> GSHMYASLTE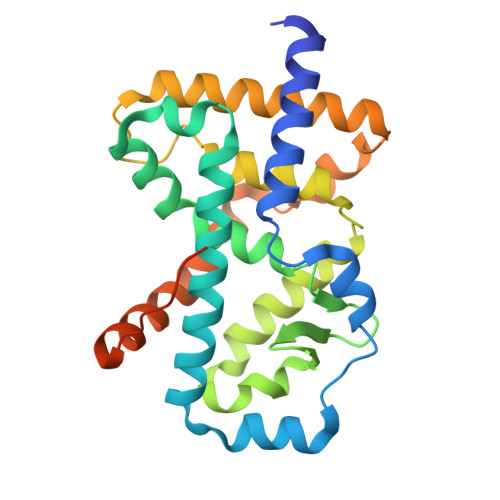IEHLVQSVCKSYRETCQLRLEDLLRQRSNIFSREEVTGYQRKSMWEMWERCAHHLTEAIQYVVEFAKRLSGFMELCQNDQIVLLKAGAMEVVLVRMCRAYNADNRTVFFEGKYGGMELFRALGCSELISSIFDFSHSLSALHFSEDEIALYTALVLINAHRPGLQEKRKVEQLQYNLELAFHHHLCKTHRQSILAKLPPKGKLRSLCSQHVERLQIFQHLHPIVVQAAFPPLYKELFSTETESPVGLSK>[4x]GSSGIVMADWLKIRGTLKSWTKLWCVLKPGVLLIYKTQKNGQWVGTVLLNACEIIERPSKKDGFCFKLFHPLEQSIWAVKGPKGEAVGSITQPLPSSYLIIRATSESDGRCWMDALELALKSG

The oxysterol-binding protein (OSBP) and its related proteins (ORP, for OSBP-related protein) have emerged as central regulators of sterol/lipid transport at the junctions formed by ER with other organelles. ORP5 and ORP8 possess the structural features of a lipid transporter: an ER anchor (TMD), a membrane targeting pleckstrin homology (PH) domain and a lipid-binding module (ORD, for OSBP-related domain). Indeed, ORP5 and ORP8, and their yeast counterparts Osh6p and Osh7p, have recently been reported to mediate the counter transport of PtdIns(4)P/phosphatidylserine (PtdSer) between the ER and plasma membrane (PM): ORP5/8 was shown to transfer PtdSer from the ER to PM, coupled with backward transport of PtdIns(4)P from PM to the ER, resulting in its hydrolysis by the phosphatase Sac114–16. Critical to the transport function of ORP5 and ORP8 is their recruitment to the ER–PM MCSs.

To understand the structural principles of ER–PM tethering by ORP5/8, the structure of the ORP8 PH domain was determined by X-ray crystallography. A distinctive feature that stands out, however, is the presence of an unusually long 25 amino acid stretch forming an extended β6–β7 loop (His209–Ser236). Comparative analysis of electrostatic surface of ORP8 PH domain with Osh3p PH domain reveals a distinct positively charged cavity, representing a putative PtdInsP-binding region. The analogous surface on the Osh3p PH domain has a neutral charge suggesting that ORP5 and ORP8 PH domains may possess a distinct PtdInsP-binding mechanism. Close inspection of the distinct positively charged cavity of ORP8 PH domain shows the amino acids forming the basic patch are lined on the β1–β2 and β5–β6 loops (non-canonical mode). Structure-based sequence alignments of related PH domain containing LTPs ORP5, ORP8, OSBP, Cert, and Osh3p establish that the putative PtdInsP residues (red inverted triangles) in ORP5 and ORP8 PH domain are not conserved in OSBP, Cert, and Osh3p. Notably the side chains (green triangles) mediating canonical PtdIns(4)P interaction with OSBP, Cert, and Osh3p are missing in ORP5 and ORP8. To confirm the importance of the non-canonical basic surface for PtdInsP binding, we designed point mutations R136Q, R179Q, and R158Q, R201Q in the ORP5 and ORP8 PH domains, respectively. Both the point mutations in ORP5 and ORP8 PH domains completely abolished the binding to PtdInsPs, confirming that ORP5 and ORP8 PH domain follows a non-canonical PtdInsP-binding regime. While most PH domains (including Osh3, OSBP) utilize the canonical PtdInsP-binding regime for PM targeting, the PH domain of ORP5/8 possesses an atypical PtdInsP-binding site that does not permit PtdIns(4)P binding.> MADNLPSDFDVIVIGTGLPESIIAAACSRSGQRVLHVDSRSY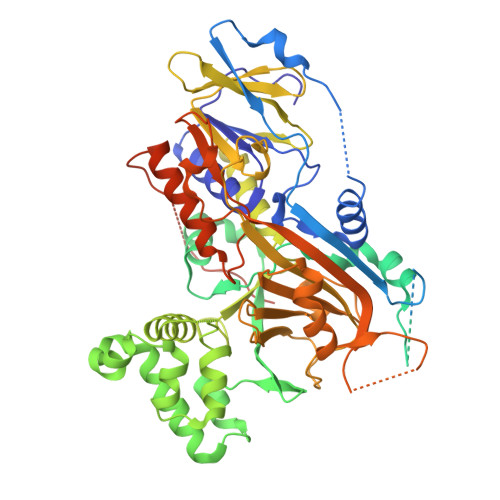YGGNWASFSFSGLLSWLKEYQENNDVVTENSMWQEQILENEEAIPLSSKDKTIQHVEVFCYASQDLHKDVEEAGALQKNHASVTSAQSAEAAEAAETSCLPTAVEPLSMGSCEIPAEQSQCPGPESSPEVNDAEATGKKENSDAKSSTEEPSENVPKVQDNTETPKKNRITYSQIIKEGRRFNIDLVSKLLYSRGLLIDLLIKSNVSRYAEFKNITRILAFREGTVEQVPCSRADVFNSKQLTMVEKRMLMKFLTFCVEYEEHPDEYRAYEGTTFSEYLKTQKLTPNLQYFVLHSIAMTSETTSCTVDGLKATKKFLQCLGRYGNTPFLFPLYGQGELPQCFCRMCAVFGGIYCLRHSVQCLVVDKESRKCKAVIDQFGQRIISKHFIIEDSYLSENTCSRVQYRQISRAVLITDGSVLKTDADQQVSILTVPAEEPGSFAVRVIELCSSTMTCMKGTYLVHLTCMSSKTAREDLERVVQKLFTPYTEIEAENEQVEKPRLLWALYFNMRDSSDISRDCYNDLPSNVYVCSGPDSGLGNDNAVKQAETLFQQICPNEDFCPAPPNPEDIVLDGDSSQQEVPESSVTPETNSETPKESTVLGNPEEPSE> ISGGDAIYSSTGRCSLGFNVRSGSTYYFLTAGHCTDGAT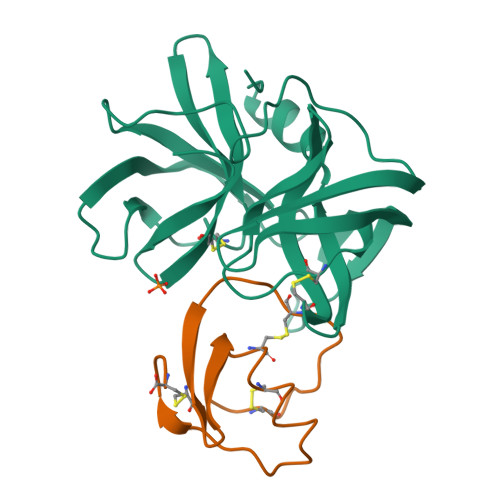TWWANSARTTVLGTTSGSSFPNNDYGIVRYTNTTIPKDGTVGGQDITSAANATVGMAVTRRGSTTGTHSGSVTALNATVNYGGGDVVYGMIRTNVCAEPGDSGGPLYSGTRAIGLTSGGSGNCSSGGTTFFQPVTEALSAYGVSVY;> VDCSEYPKPACTYEYRPLCGSDNKTYGNKCNFCNAVVESNGTLTLSHFGKC NarK is highly expressed during anaerobic growth in the presence of nitrate, and plays a central role in nitrate uptake, while NarU has important functions during severe nutrient starvation or slow growth. In this work, we demonstrate that NarK is a nitrate/nitrite antiporter, using an in vitro reconstituted system. The overall structures of NarK in both the occluded and inward-open states adopt a canonical MFS-fold with 12 TM helices, with TM1–TM6 and TM7–TM12 forming the N and C bundles, respectively. The substrate-binding site is located at the interface between the N and C bundles, in the middle of the TM segment.

In the nitrate-bound, inward-open structure, a triangular electron-density peak of a nitrate ion was also observed in the substrate-binding site. However, we found several differences in the recognition manner of the substrate nitrate, as compared with that in the occluded state. In the inward-open structure, the bending of TM7, TM10 and TM11 leads to a slight movement of the side chains of Y263 in TM7 and R305 in TM8, away from the centre of the transporter. As a result, the following changes were observed in the interactions in Sites A and B. In Site A, the distance between one oxygen atom of the nitrate ion and the R89 guanidinium group is increased from 2.7 to 3.1 Å. In Site B, the distance between the nitrate ion and the Y263 phenol group is increased from 2.4 to 3.9 Å, and only one oxygen atom is within hydrogen-bonding distance with the Y263 phenol group. These changes in Sites A and B increase the volume of the substrate-binding site in the inward-open state structure (37.6 and 50.5 Å3 for the occluded and inward-open structures, respectively). Taken together, the overall structural change in the transition from the nitrate-bound occluded to the inward-open state, including the bending of TM7, TM10 and TM11, induces the movement of Y263 and R305 in Site B, which enlarges the volume of the substrate-binding site. This change in the substrate-binding site may result in decreased substrate affinity in the inward-open state, thereby facilitating substrate release towards the cytoplasmic side. In contrast to their conformations in the present occluded structure of NarK, in the inward-open structure, TM7, TM10 and TM11 in the C bundle are bent at the conserved Gly residues. As a result, none of the interactions in layers C1, C2 and C3 is formed. The transport pathway is thereby formed between the N and C bundles, and the substrate-binding site is accessible from the cytosolic side.

> MSHSSAPERATGAVITDWRPEDPAFWQQRGQRIASRNLWISVPCLLLAFCVWMLFSAVAVNLPKVGFNFTTDQLFMLTALPSVSGALLRVPYSFMVPIFGGRRWTAFSTGILIIPCVWLGFAVQDTSTPYSVFIIISLLCGFAGANFASSMANISFFFPKQKQGGALGLNGGLGNMGVSVMQLVAPLVVSLSIFAVFGSQGVKQPDGTELYLANASWIWVPFLAIFTIAAWFGMNDLATSKASIKEQLPVLKRGHLWIMSLLYLATFGSFIGFSAGFAMLSKTQFPDVQILQYAFFGPFIGALARSAGGALSDRLGGTRVTLVNFILMAIFSGLLFLTLPTDGQGGSFMAFFAVFLALFLTAGLGSGSTFQMISVIFRKLTMDRVKAEGGSDERAMREAATDTAAALGFISAIGAIGGFFIPKAFGSSLALTGSPVGAMKVFLIFYIACVVITWAVYGRHSKKLESSGENLYFQG>[16x]SHHHHHHGGMSGLNATMPLSCSKNNSHHYIQVRNDTGLELTLTNTSLLDHKFCNLSDAHKRNLYDKALMSIVTTFHLNIPNF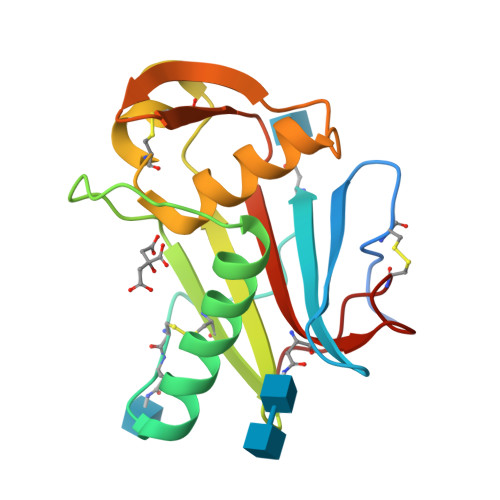NQYEVMSCDFNGGKITVQYNLSHSSYVDAANHCGTIANGIMDTFRRMYWSNALSPSEYISGTTCIQTAYQYLIIQNTTWEDHCVFSRPS Here, we report that a critical glycine residue (Gly463) dominates the motion of threonyl-tRNA synthetase (ThrRS) and the sensitivity of the enzyme to antibiotics. The natural product Obafluorin (OB) is a potent inhibitor of bacterial threonyl-tRNA synthetase (ThrRS). Our previous work showed that OB covalently binds to ThrRS, forming an ester bond with a tyrosine residue in the catalytic center via the highly strained β-lactone ring, making OB the first covalent aaRS inhibitor with demonstrated crystal structures. The binding of OB induces a large conformational change in ThrRS.

We noticed that Gly463 and Leu489 are two strictly conserved residues in the ThrRS proteins, but they are replaced by a serine and a methionine in the ObaOs, respectively. Therefore, the mutation of Leu489 to a methionine does not confer resistance of EcThrRS to OB. In contrast, OB showed poor activity against EcThrRS_G463S, with 5 μM OB inhibiting only approximately 10% of the activity of EcThrRS_G463S, indicating that mutating Gly463 to a serine renders EcThrRS resistant to OB. In contrast, cocrystallizing 300 μM EcThrRS_G463S protein with 600 μM OB did not result in an EcThrRS_G463S–OB complex structure. No electron density of OB was observed in the catalytic pocket of EcThrRS_G463S under this condition. The active pocket of this structure has neither an OB nor substrate molecules, so it is in an “apo state”. The conformation in this state is similar to the “adenylation state” of the EcThrRS_Y462F–ATP complex structure we determined earlier, but slightly wider. This structure also indicates that although G463S weakens ThrRS binding to OB, it does not disrupt the active conformation of ThrRS. In the EcThrRS_G463S structure, the hydroxyl group of Ser463 is 5.0 Å away from the phenolic hydroxyl group of Tyr462, which attacks the lactone structure of OB and forms a covalent bond with it. Thus, the sidechain of Ser463 is too short to clash with the presumably bound OB and it is also unlikely that Ser463 will directly affect the nucleophilicity of Tyr462 and prevent it from forming a covalent bond with OB. However, the motion of these two groups was positively correlated in the MD trajectories of the EcThrRS_G463S mutant, suggesting that the pocket of this mutant is relatively rigid.

>[2x]MRDHRKIGKQLDLYHMQEEAPGMVFWHNDGWTIFRELEVFVRSKLKEYQYQEVKGPFMMDRVLWEKTGHWDNYKDAMFTTSSENREYCIKPMNCPGHVQIFNQGLKSYRDLPLRMAEFGSCHRNEPSGSLHGLMRVRGFTQDDAHIFCTEEQIRDEVNGCIRLVYDMYSTFGFEKIVVKLSTRPEKRIGSDEMWDRAEADLAVALEENNIPFEYQLGEGAFYSPKIEFTLYDCLDRAWQCGTVQLDFSLPSRLSASYVGEDNERKVPVMIHRAILGSMERFIGILTEEFAGFFPTWLAPVQVVIMNITDSQSEYVNELTQKLSNAGIRVKADLRNEKIGFKIREHTLRRVPYMLVCGDKEVESGKVAVRTRRGKDLGSMDVNEVIEKLQQEIRSRSLKQLEELEHHHHHH The discoidin domain receptors (DDRs), DDR1 and DDR2, are unique among the receptor tyrosine kinases (RTKs) in being activated by interaction with the extracellular matrix. A single transmembrane helix links to the cytoplasmic domain, where a larger JM region precedes the catalytic C-terminal kinase domain. Overall, DDR1 displays the classical bilobal architecture of a tyrosine kinase. As observed for ABL, both type II inhibitors induce an inactive conformation of DDR1 characterized by a “DFG-Asp out, αC-Glu in” configuration.

Ponatinib is a third-generation TKI developed for the treatment of CML patients with resistance to imatinib. DDR1 was monomeric in the imatinib complex, consistent with its size-exclusion profile, whereas the ponatinib complex formed a crystallographic dimer with an additional ponatinib molecule bound at the dimer interface. By design, ponatinib binds at the same site with the loss of one hydrogen bond owing to the ethynyl linker, which removes any polar interaction with the gatekeeper residue Thr701. Hinge interactions are made instead by an imidazo[1,2b]pyridazine head group, which establishes the hydrogen bond with Met704. In addition to the remaining four hydrogen bonds, there are extensive hydrophobic interactions across the DDR1 pocket, although the π–π interaction with Phe785 is broken. The added trifluoromethyl group occupies the pocket vacated by the inverted DFG motif and forms favorable hydrophobic contacts with Leu679, Ile684, Ile685, Leu757 and Ile782. ITC measurements suggested that the ponatinib interaction was slightly stronger than imatinib, with a calculated KD of 1.3 nM. Similar potency was observed in U2OS cells, where ponatinib inhibited collagen-induced DDR1 autophosphorylation with an EC50 of 2.5 nM. Interesting in this respect is the ponatinib molecule that stabilizes the crystallographic dimer in the kinase–inhibitor complex. While we have not investigated this effect in solution, it may be of relevance for the full-length DDR1 and DDR2 receptors, which form constitutive homodimers at the cell surface.

>SMPRVDFPRSRLRFKEKLGEGQFGEVHLCEVDSPQDLVSLDFPLNVRKGHPLLVAVKILRPDATKNARNDFLKEVKIMSRLKDPNIIRLLGVCVQDDPLCMITDYMENGDLNQFLSAHQLEDKAAEGAPGDGQAAQGPTISYPMLLHVAAQIASGMRYLATLNFVHRDLATRNCLVGENFTIKIADFGMSRNLYAGDYYRVQGRAVLPIRWMAWECILMGKFTTASDVWAFGVTLWEVLMLCRAQPFGQLTDEQVIENAGEFFRDQGRQVYLSRPPACPQGLYELMLRCWSRESEQRPPFSQLHRFLAEDALNTV[2x]> MEKYF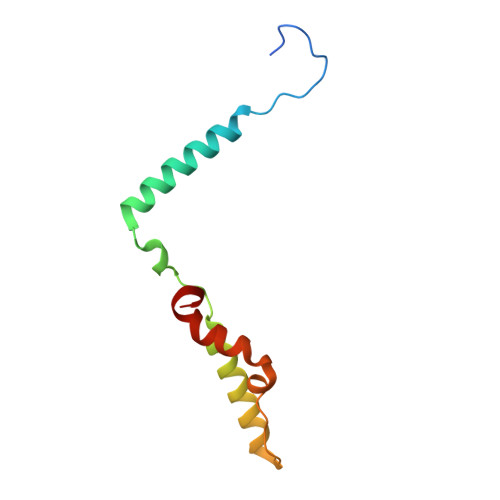GNAYRGDPGVPHADADRFVNIWIGSAAFSVLTWVNPYMWQLSNQFNYHDKWMLFEQYHWKKARAKKQPYEFKWNKIPKEVRDSYYYNWPVYFP> MLLAALLAALVARTTLGADVDAVPAPTFPPPAYPYTESWQLTLTTVPSPFVGPADVYHTRPLEDPCGVVALISDPQVDRLLNEAVAHRRPTYRAHVAWYRIADGCAHLLYFIEYADCDPRQVFGRCRRRTTPMWWTPSADYMFPTEDELGLLMVAPGRFNEGQYRRLVSVDGVNILTDFMVALPEGQECPFAR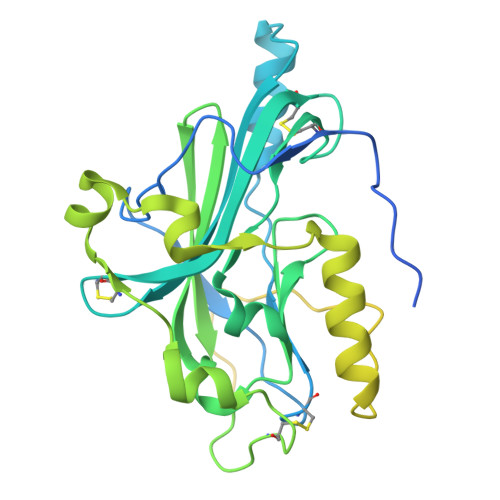VDQHRTYKFGACWSDDSFKRGVDVMRFLTPFYQQPPHREVVNYWYRKNGRTLPRAYAAATPYAIDPARPSAGSPRPRPRPRPRPRPKPEPAPATPAPPDRLPEPATRDHAAGGRPTPRPPRPETPHRPFAPPAVVPSGWPQPAEPFQPRTPAAPGVSRHRSVIVGTGTAMGALLVGVCVYIFFRLRGAKGYRLLGGPADADELKAQPGP>MNITKPFPLPTGYFGIPLGLAALSLAWFHLENLFPAARMVSDVLGIVASAVWILFILMYAYKLRYYFEEVRAEYHSPVRFSFIALIPITTMLVGDILYRWNPLIAEVLIWIGTIGQLLFSTLRVSELWQGGVFEQKSTHPSFYLPAVAANFTSASSLALLGYHDLGYLFFGAGMIAWIIFEPVLLQHLRISSLEPQFRATMGIVLAPAFVCVSAYLSINHGEVDTLAKILWGYGFLQLFFLLRLFPWIVEKGLNIGLWAFSFGLASMANSATAFYHGNVLQGVSIFAFVFSNVMIGLLVLMTIYKLTKGQFFLK[3x]

The SLAC1 homolog, HiTehA, although not completely biochemically characterized, is identified as a transporter protein involved in tellurite resistance and adaptation to environmental stresses, highlighting its role in bacterial survival through regulating solute concentrations. HiTehA is a trimeric protein; each monomer comprises 10 transmembrane helices (TMs) connected by short extracellular loops and slightly longer intracellular loops; a short helix is part of the loop connecting TM2. The ion channel architecture features a distinctive organization: the pore-forming helices are positioned at odd-numbered TMs, while the even TMs collectively form an outer shell. This outer shell contributes significantly to the overall stability and functionality of the channel, potentially playing a pivotal role in sensing environmental changes, responding to stimuli, and regulating the opening and closing dynamics of the channels.

We successfully elucidated the structures of all four samples with an average resolution of 3 Å. The HiTehA purified using GDN achieved the highest resolution of 2.9 Å, followed by those purified with DDM and LMNG at resolutions of 3.1 Å, and OG at 3.2 Å, as detailed in Table 1 and Figure S1. The four structures of HiTehA closely align, revealing a minimal root-mean-square deviation (r.m.s.d.) of 0.13 Å for all atoms, except for the sample purified in DDM, which showed a slightly higher deviation of 0.26 Å. This discrepancy may be attributed to distinct folding patterns in the intracellular loops between TM6 and TM7. In general, the structural integrity of the trimeric arrangement remains unaffected using four different detergents during protein purification. Remarkably, none of the detergents tested appear to induce any significant alteration in the position of the gating Phe262 located on TM9. This observation underscores the robustness of the trimeric structure and the stability of key functional elements within HiTehA, even under varying detergent conditions. The identification of a linear density within the channel cavity across all detergent conditions suggests this cavity can be occupied either by detergent molecules or by other hydrophobic molecules such as co-purified lipids.> MGHHHHHHPSGVKTENNDHINLKVAGQDGSVVQFKIKRHTPLSKLMKAYCERQGLSMRQIRFRFDGQPINETDTPAQLEMEDEDTIDVFQQQTGGCMDPPSDAESPVTDDGFTLQLSQDASLCPSNSGTFSIIDVASDRRLFNTFIKEWKTKERYSLALACEKREHIQQPEGEIGGKHKRAPAARQKLNRTDGFPVRDSDGLVLIGLSVCWGARDSYYISLQQEQSKGLSSSLAPPPLDDDLPVSERLGQVRSCLSRPSAGLRGGVVVTYDIIQVYKTLVLSCGISLAGNCEDPKVACWLLDPGSEERTLPNMVTVYCPEELPLLDGLGSAHAHCPRVRAATKSVLVHAVMNHLTGLLEKDSMLDLFRSIEMPSQVCLALLELNGVGFSVEECERQKHVMQAKLTALESQAYNLAGHSFSLTSIDDIAQVLFLELHLPPNGDVGGSKSKKTLGYTRRGGGRVRLGKQFSTTKDILEKLRPLHPLPGVILEWRRITNALTKVVFPLQREKQYHPTLAMDRIYPIAQTHTATGRVSFTEPNIQNVPKDFEICMPTVVGESPPSQNGCQMTTKPGKNRRSVAPSVTGGAAEQGPAFSVSMRHAFVPFSGGMILAADYSQLELRVLAHLSKDQRLLQVLNGGADVFRCIAAEWKGVDPETVNDSLR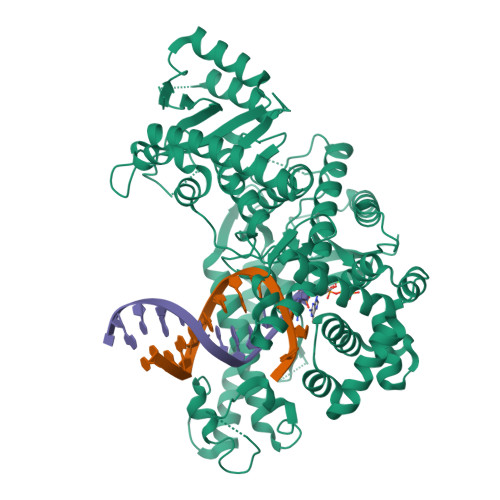QQAKQICYGIIYGMGAKSLGEQMGVEENDAACYIESFKARYKGINAFLKETVKNCIKNGYVQTLMGRRRYLPGISNTNTHIKAHAERQAVNTTVQGSAADIVKLATVNIQKRLRKTYPTAPLSHQHTHSGTSQYRAGTSHLRGAFFVLQLHDELIYETREEDLIQVAQIVKREMESAVKLYVKLKAKVKVGPSWGNLQDLDL>[2x]MSEPESLMGKLTTHILDLTCGKPAANVKIGLKRLGESIMKEVY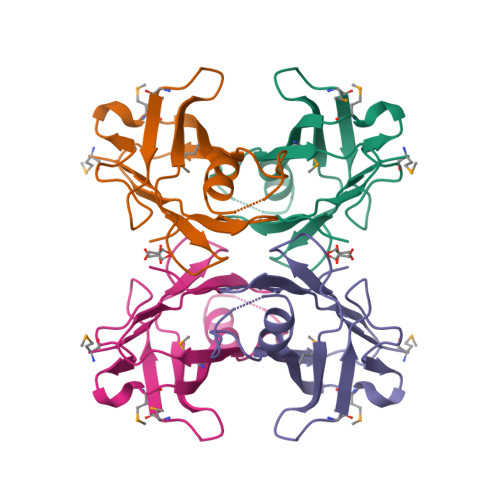TNNDGRVDVPLLAGEELMSGEYVMEFHAGDYFASKNMNAADQPFLTIVTVRFQLADPDAHYHIPLLLSPFGYQVYRGS1-((2-HYDROXYETHOXY)METHYL)-5-(3-(BENZYLOXY)BENZYL)-6-HYDROXYPYRIMIDINE-2,4(1H,3H)-DIONE 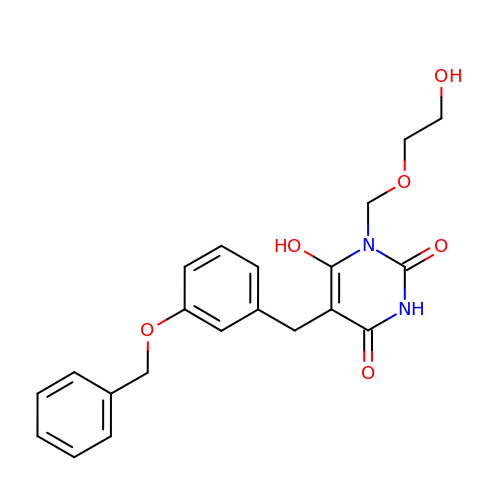| C21 H22 N2 O6 | CAWXCABXSPTFRN-UHFFFAOYSA-N In budding yeast, single‐stranded DNA is coated by replication protein A (RPA) following DNA end resection, and DNA–RPA complexes are then SUMO‐modified by the E3 ligase Siz2 to promote repair. In budding yeast, the response to genotoxic stress is triggered by the formation of single‐stranded DNA and leads to protein group modification by SUMO in a manner that is dependent on the SUMO E3 ligase Siz2 (Cremona et al, 2012; Psakhye & Jentsch, 2012). The SAP domain of Siz2 binds DNA duplexes and makes a key contribution to this process as highlighted by models and a crystal structure of Siz2 and by assays performed using protein mutants. Our results provide insights on how DNA architecture scaffolds a substrate and E3 ligase to promote SUMO modification in the context of DNA repair.

A fragment of Siz2 encompassing the PINIT and SP‐RING domains is inactive toward RPA. This was unexpected because an equivalent fragment of Siz1 retains activity and specificity toward substrates such as PCNA in vitro. We queried if this fragment of Siz2 differs in any substantive manner from Siz1 relative to its substrate, E2 or SUMO binding surfaces by obtaining a crystal structure of this fragment at a resolution of 2.65 Å. The structure includes two protomers in the asymmetric unit that share high structural similarity (0.7 Å rmsd over 261 Cα atoms). The structure of Siz2 includes the N‐terminal PINIT domain as well as the SP‐RING and SP‐CTD domains for structures of Siz1. The structures of Siz1 and Siz2 can be superposed with an RMSD of 2.2 Å rmsd over 256 Cα atoms. The largest overall deviations arise due to differing orientations of the PINIT domains relative to the SP‐RING domains and to different conformations of the 210‐220 loop within the PINIT domain, so if the PINIT and SP‐RING domains are aligned separately without the 210‐220 loop, they superpose with a 1.5 Å rmsd over 124 Cα atoms–sequence identity of 41% or a 1.0 Å rmsd over 123 Cα atoms–sequence identity of 63%, respectively. The amino acid residues that are important for contacting the E2 and SUMO in Siz1 are generally well conserved between Siz2 and Siz1. The Siz2 structure suggests that its PINIT and SP‐RING domain are correctly folded, with the latter appearing competent for E2 and SUMO binding. These observations, combined with our inability to detect activities for this fragment, underscore a role for dsDNA, the SAP domain, and ssDNA in templating a complex to promote RPA binding and modification.

>SLFTSPFYKPIVQIPDANKKLKQSAGRGCTKMKFKVSKSNHDLLKSNKSYKLYLFSGFSIPFIYETVGHEAIDFPYPCELVFNGTKLEDNVKGLKKQNGTGNPANLTPYLKVPTEMNHLDLHYLNIDKEYSISCFIVEVFSPEALLGKILKRPKIIKQATTAYIKRTLNEQDDDDIITTSTVLSLQCPISCTRMKYPAKTDQCKHIQCFDALWFLHSQSQVPTWQCPICQHPIKFDQLKISEFVDNIIQNCNEDVEQVEISVDGSWKPI[2x]> FQKK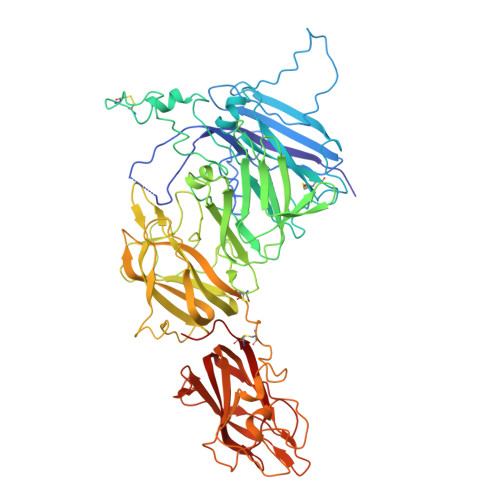TRHYFIAAVERLWDYGMSSSPHVLRNRAQSGSVPQFKKVVFQEFTDGSFTQPLYRGELNEHLGLLGPYIRAEVEDNIMVTFRNQASRPYSFYSSLISYEEDQRQGAEPRKNFVKPNETKTYFWKVQHHMAPTKDEFDCKAWAYFSDVDLEKDVHSGLIGPLLVCHTNTLNPAHGRQVTVQEFALFLTIFDETKSWYFTENMERNCRAPCNIQMEDPTFKENYRFHAINGYIMDTLPGLVMAQDQRIRWYLLSMGSNENIHSIHFSGHVFTVRKKEEYKMALYNLYPGVFETVEMLPSKAGIWRVECLIGEHLHAGMSTLFLVYSNKCQTPLGMASGHIRDFQITASGQYGQWAPKLARLHYSGSINAWSTKEPFSWIKVDLLAPMIIHGIKTQGARQKFSSLYISQFIIMYSLDGKKWQTYRGNSTGTLMVFFGNVDSSGIKHNIFNPPIIARYIRLHPTHYSIRSTLRMELMGCDLNSCSMPLGMESKAISDAQITASSYFTNMFATWSPSKARLHLQGRSNAWRPQVNNPKEWLQVDFQKTMKVTGVTTQGVKSLLTSMYVKEFLISSSQDGHQWTLFFQNGKVKVFQGNQDSFTPVVNSLDPPLLTRYLRIHPQSWVHQIALRMEVLGCEAQDLY> MDEFEMIKRNTSEIISEEELREVLKKDEKSAGIGFEPSGKIHLGHYLQIKKMIDLQNAGFDIIIELADLHAYLNQKGELDEIRKIGDYNKKVFEAMGLKAKYVYGSEWMLDKDYTLNVYRLALKTTLKRARRSMELIAREDENPKVAEVIYPIMQVN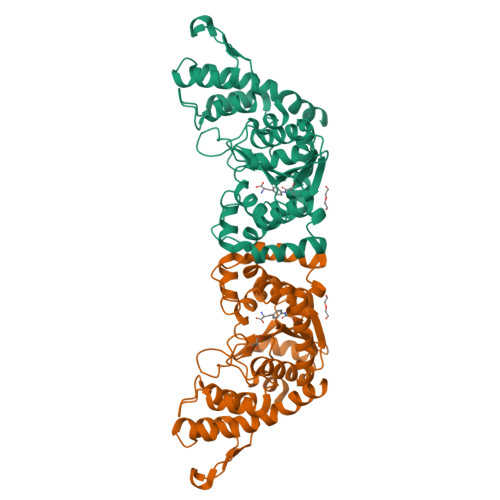SIHYKGVDVAVGGMEQRKIHMLARELLPKKVVCIHNPVLTGLDGEGKMSSSKGNFIAVDDSPEEIRAKIKKAYCPAGVVEGNPIMEIAKYFLEYPLTIKRPEKFGGDLTVNSYEELESLFKNKELHPMDLKNAVAEELIKILEPIRKRLLEHHHHHH> EASCGSPPPILNGRISYYSTPIAVGTVIRYSCSGTFRLIGEKSLLCITKDKVDGTWDKPAPKCEYFNKYSSCPEPIVPGGYKIRGST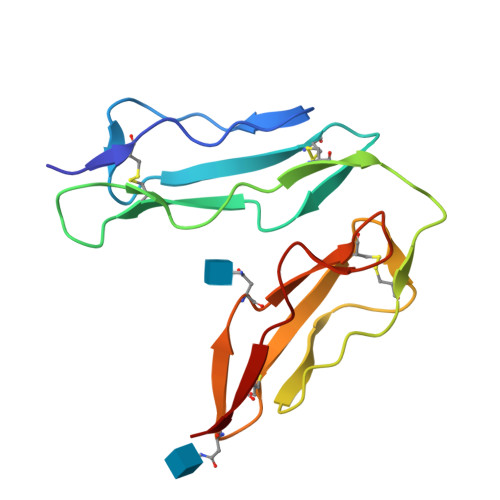PYRHGDSVTFACKTNFSMNGNKSVWCQANNMWGPTRLPTCVSI>[2x]MTINNDPMRDAIVDTAVELAAHTSWEA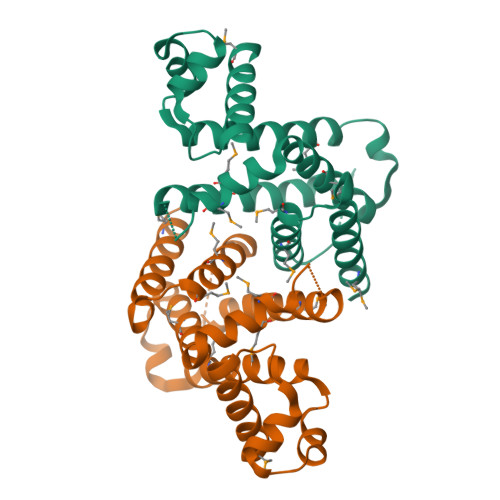VRLYDIAARLAVSLDEIRLYFREKDELIDAWFDRADSRMLKEAESAGFLDLVASERIHHLIMIWLDALAVQRKVTRQMIMSKLEFGHIHIQIPAVMRVSRTVQWVREAAQRDATFMRRALEESTLTTIYLMTFFFWMRDESENSRHTRQFLKRHLTMAAWLGQKVYGKDPEKSTVPHKQQIPLQFD>[4x]MGSDKIHHHHHHMIRAGIIGATGYTGLELVRLLKNHPEAKIT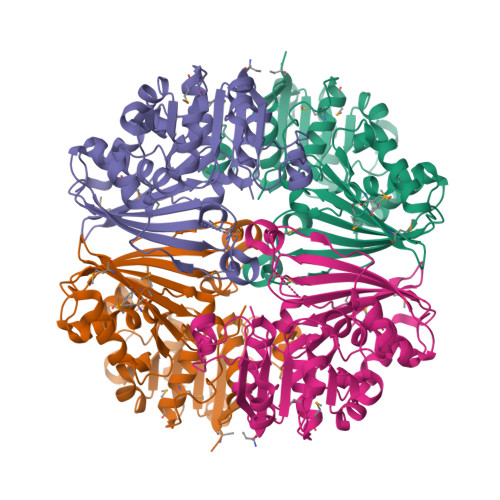YLSSRTYAGKKLEEIFPSTLENSILSEFDPEKVSKNCDVLFTALPAGASYDLVRELKGVKIIDLGADFRFDDPGVYREWYGKELSGYENIKRVYGLPELHREEIKNAQVVGNPGCYPTSVILALAPALKHNLVDPETILVDAKSGVSGAGRKEKVDYLFSEVNESLRPYNVAKHRHVPEMEQELGKISGKKVNVVFTPHLVPMTRGILSTIYVKTDKSLEEIHEAYLEFYKNEPFVHVLPMGIYPSTKWCYGSNHVFIGMQMEERTNTLILMSAIDNLVKGASGQAVQNMNIMFGLDETKGLEFTPIYP>[4x]DIKVTPGTSELVEQ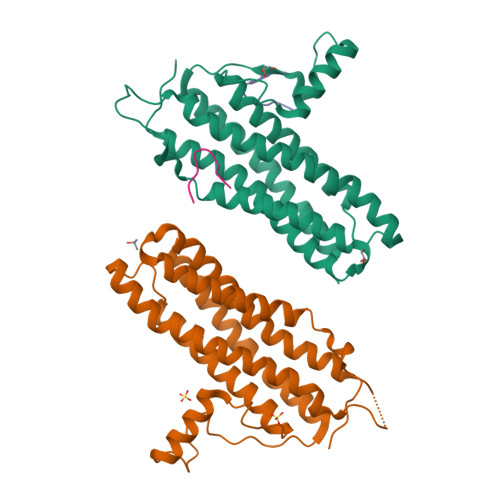ILALLSRYLSSYIHVLNKFISHLRRVATLRFERTTLIKFVKKLRFYNDSVLSYNASEFINEGKNELDPGADSFDKVILPIASMFVKCVETFDLLNYYLTQSLQKEILSKTLNEDLTLTAESILAIDDTYNHFVKFSQWMIESLRIGSNLLDLEVVQFAIKSADEDGTNIGETDNIFLQEILPVNSEEEFQTLSAAWHSILDGKLGALDEEFDVVATKWHD;>RSFYTASPLLSSGSIPKSASPVLPGVKRTASVR[4x]>MKDLSHYGPALCVKFYNDYVLAGYGPFIHVYDYHSATLINKCRLFHYNKVHGLSLSSEGKILAYGARSVTIVELEDVLKKESLVDFERINSDWITGATFSFDNLQIYLLTCYNKVLICDLNCEVLFRKSLGGERSILYSGIIKVFGPDKVYVNAGTVMGGVIIWDLFSETKIHNLLGHEGSIFYVNLSNNGRYVASCSDDRSIRLWDLETGKQLSVGWSHTARIWNLMFFDNDSKLISVSEDCTCRVWNIIESRENVAELSISNVYEVHLIKSIWGVDVKDDEMIAVTSGNDGRLKLIDLLQLKRHGDEETSFSLDDIAKQCGDIFEKNESIKGFQWFSFGVIAITSLGKILKYSDVTKQWKLLLTNEKFNSYPITNGIQTQNIAVFSNNKSDILLIKFSKDSADIIETEEFHLDELSKTNNCLVTEYDDDSFLLTLQSPNPREKFVCLEISLQNLKIKSKHCFNKPENFSSSCLTSFRNHILVGSRFSTLVIYNLLDESEEPFIIRRLSPGDTTTSIEFVEDKDNSAVFSVTNRDGYYVFIELTKNSLEEGPYRLSYKVLHSNKMMKGFLEGAFFNSKGEYITYGFKSSLFYLYNETNCYELASEVCGGSHRLWNLAKITDGHVLMYIKASRFHLRKIYNSIVPETLENGVHGREIRDISICPVSNTNTNDNFKDGHIFCTASEDTTIKLGYFNNRTGKVQNFWTQRKHVSGLQRCQFINHKLMISSSAREELFLWELNDKYNKRPYMTIRQALPVSTNNSDLRIMDFDVKFISQSGDFLLVTVYSDSTIKIWHYRENQNKFDLIMQGRYKTCCLFNVVFIALKEELLVVISPTDGHLVVYNITEYVPFSVDPISGDLVDHKLDATISNLPAPVAQLPVHQSGVKSLDYVANATRTSATILTGGDDNGLGLSNLKLDDSNKVTLKTSDFIAA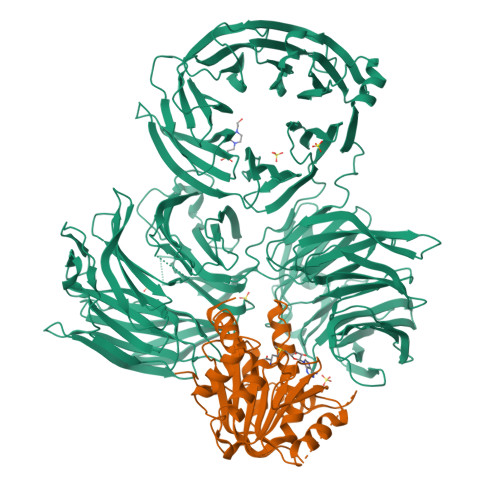AASSTITSGMLINGGKEVITTSVDQVIRAWEITAGKLSLVDKKRTTVADTGSLEIISNDEDADSEKTLLIGGVGLSIWKKLEVLFQGPSHHHHHH[2x];>MGKSSKDKRDLYYRKAKEQGYRARSAFKLLQLNDQFHFLDDPNLKRVVDLCAAPGSWSQVLSRKLFDESPSSDKEDRKIVSVDLQPMSPIPHVTTLQADITHPKTLARILKLFGNEKADFVCSDGAPDVTGLHDLDEYVQQQLIMSALQLTACILKKGGTFVAKIFRGRDIDMLYSQLGYLFDKIVCAKPRSSRGTSLEAFIVCLGYNPPSNWTPKLDVNTSVDEFFQGCFLNKLCISDKLSHWNEEERNIAEFMACGSLQSFDSDATYHDLPSSVAGTSSSLDPVQSPTNPPYKKALELKRSGKLTRSVLEVLFQGPSHHHHHH[2x]> MKNVGFIGWRGMVGSVLMDRMSQENDFENLNPVFFTTSQAGQKAPVFGGKDA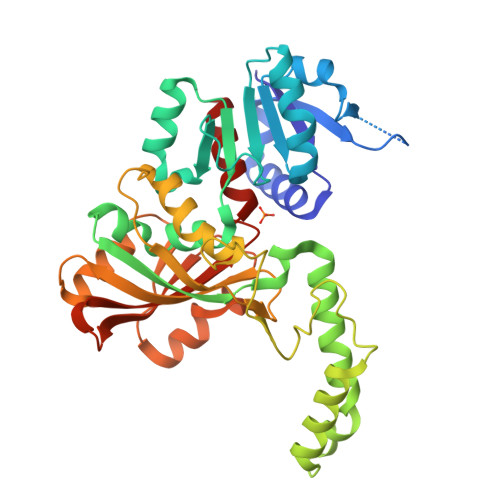GDLKSAFDIEELKKLDIIVTCQGGDYTNEVYPKLKATGWDGYWVDAASALKMKDDAIIVLDPVNQHVISEGLKKGIKTFVGGNCTVSLMLMAIGGLFEKDLVEWISVATYQAASGAGAKNMRELLSQMGLLEQAVSSELKDPASSILDIERKVTAKMRADNFPTDNFGAALGGSLIPWIDKLLPETGQTKEEWKGYAETNKILGLSDNPIPVDGLCVRIGALRCHSQAFTIKLKKDLPLEEIEQIIASHNEWVKVIPNDKEITLRELTPAKVTGTLSVPVGRLRKLAMGPEYLAAFTVGDQLLWGAAEPVRRILKQLVA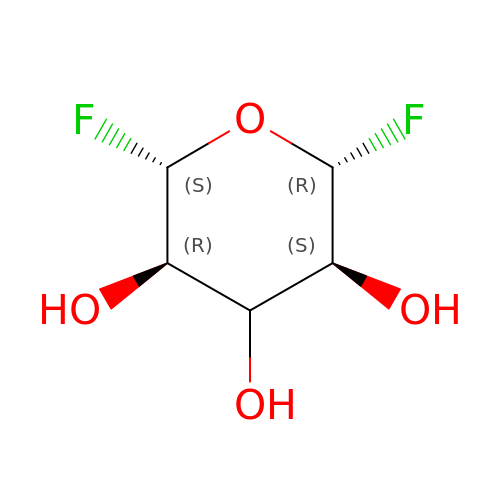(2R,3S,5R,6S)-2,6-DIFLUOROOXANE-3,4,5-TRIOL | C5 H8 F2 O4 | QCYATGUEQPTSRF-IYJRPRHRSA-N> EVTVPDALKDRIALKKTARQLNIVYFLGSDTEPVPDYERRLSELLLYLQQFYGKEMQRHGYGARSFGLDIKSPGRVNIIEYKAKNPAAHYPYENGGGWKAAQELDEFFKAHPDRKKSQHTLIIMPTWNDEKNGPDNPGGVPFYGMGRNCFALDYPAFDIKHLGQKTREGRLLTKWYGGMAHELGHGLNLPHNHQTASDGKKYGTALMGSGNYTFGTSPTFLTPASCALLDACEVFSVTPSQQFYEGKPEVEVGDVAISFKGDQILVSGNYKSPQTVKALNVYIQDPPYAVNQDYDAVSFSRRLGKKSGKFSMKIDKKELEGLNNNEFRISLMFILANGLHMQKHFTFHWDALQDYRDGSKSGSGHHHHHH

Here we focus on OgpA from A. muciniphila, a recently discovered O-glycopeptidase that exclusively hydrolyzes the peptide bond N-terminal to serine or threonine residues substituted with an O-glycan. OgpAWT comprises two domains from the N- to the C-terminus: (i) a catalytic domain (residues 25–262) followed by (ii) a β-sandwich domain (residues 263-385). Interestingly, a Zn2+ atom coordinates with the side chains of three histidine residues, H205, H209, and H215, a highly conserved triad among metalloproteases. A glutamate residue, E206, is well-positioned to act as a general base/acid during catalysis.

The crystal structure of full-length OgpA in its unliganded form was solved using zinc single-wavelength anomalous dispersion (Zn-SAD). The high quality of the electron density maps allowed the trace of residues 27–380 (OgpAWT1) and 25 to 382 (OgpAWT2). The overall protein scaffold and the conformation of the OgpAWT1 and OgpAWT2 were essentially preserved (root mean square deviation, r.m.s.d., of 0.37 Å for 350 residues). However, the connecting loop α4–α5 (loop 9; residues 227–246) is unstructured in OgpAWT2 whereas in OgpAWT1 displays a short α-helix. Furthermore, we were unable to fully model the β7–β8 connecting loop (loop 12; residues 309–320) on OgpAWT2 crystal structure because it is disordered. A close inspection of the two crystal structures revealed that the protein crystallized as a monomer. The first β-sheet of the antiparallel β-sandwich domain consists of four β-strands with topology β6–β7–β8–β11, whereas the second β-sheet comprises four β-strands with topology β13–β12–β9–β10, with an overall size of 39 × 28 × 19 Å (“Methods” section). Both domains are separated by a long and open groove that runs parallel to the protein surface where the active site is located.> MSEIVVSKFGGTSVADFDAMNRSADIVLSDANVRLVVLSASAGITNLLVALAEGLEPGERFEKLDAIRNIQFAILERLRYPNVIREEIERLLENITVLAEAAALATSPALTDELVSHGELMSTLLFVEILRERDVQAQWFDVRKVMRTNDRFGRAEPDIAALAELAALQLLPRLNEGLVITQGFIGSENKGRTTTLGRGGSDYTAALLAEALHASRVDIWTDVPGIYTTDPRVVSAAKRIDEIAFAEAAEMATFGAKVLHPATLLPAVRSDIPVFVGSSKDPRAGGTLVCNKTENPPLFRALALRRNQTLLTLHSLNMLHSRGFLAEVFGILARHNISVDLITTSEVSVALTLDTTGSTSTGDTLLTQSLLMELSALCRVEVEEGLALVALIGNDLSKACGVGKEVF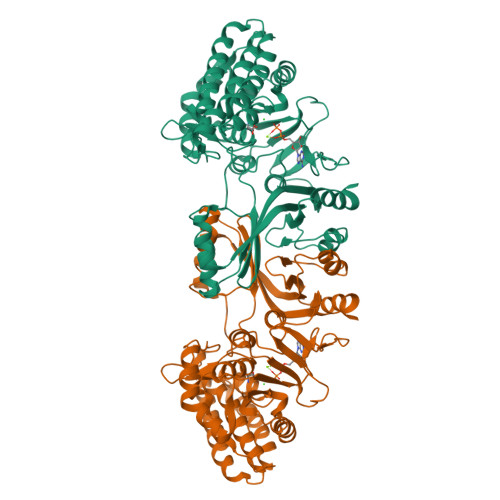GVLEPFNIRMICYGASSHNLCFLVPGEDAEQVVQKLHSNLFE[(1R,2S)-2-(2-hydroxybenzene-1-carbonyl)cyclopentyl]acetic acid 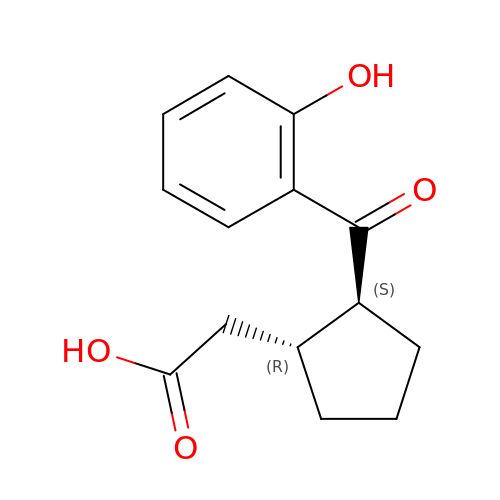| C14 H16 O4 | LULBZYDRYZGRST-ZJUUUORDSA-N> VLED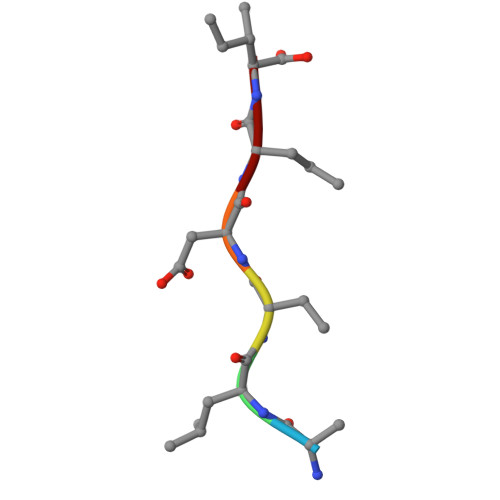RI>[2x]GSAMASNAVLYKSNHNVVY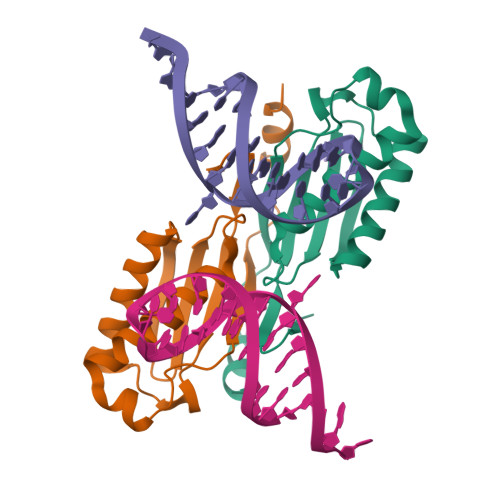SCKYHIVWCPKYRRKVLVGAVEMRLKEIIQEVAKELRVEIIEMQTDKDHIHILADIDPSFGVMKFIKTAKGRSSRILRQEFNHLKTKLPTLWTNSCFISTVGGAPLNVVKQYIENQQNSNRPKQKEKWKSYVDNLQTKAL>MTSAEMTSPNNNSEHQAIAKMRTMIEGFDDISHGGLPIGRSTLVSGTSGTGKTLFSIQFLYNGIIEFDEPGVFVTFEETPQDIIKNARSFGWDLAKLVDEGKLFILDASPDPEGQEVVGGFDLSALIERINYAIQKYRARRVSIDSVTSVFQQYDASSVVRRELFRLVARLKQIGATTVMTTERIEEYGPIARYGVEEFVSDNVVILRNVLEGERRRRTLEILKLRGTSHMKGEYPFTITDHGINIFPLGAMRLTQRSSNVRVSSGVVRLDEMCGGGFFKDSIILATGATGTGKTLLVSRFVENACANKERAILFAYEESRAQLLRNAYSWGMDFEEMERQNLLKIVCAYPESAGLEDHLQIIKSEINDFKPARIAIDSLSALARGVSNNAFRQFVIGVTGYAKQEEITGLFTNTSDQFMGAHSITDSHIAEITDTIILLQYVEI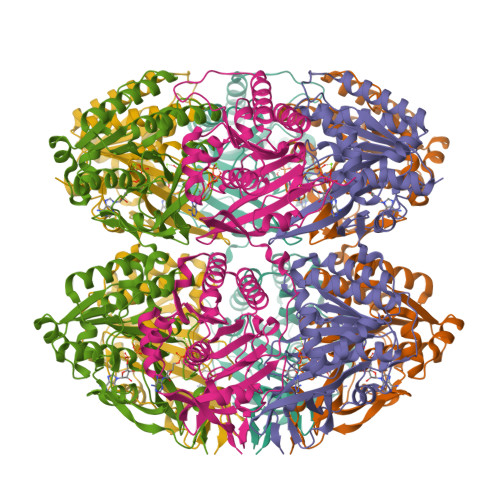RGEMSRAINVFKMRGSWHDKAIREFMISDKGPDIKDSFRNFERIISGSPTRITVDEKSELSRIVRGVQEKGPES[6x]> MFIKPGRCPKPAVQEDFDAARYLGVWYDIQRLPNKFQKGECATATYSLSPGVGFSVFNRERLANGTIKSVIGSAIAEDPCEPAKLQFFHENAAPVPYWVLSTDYDNYALVYSCINEGASHAAYASIVSRQPTLPEETIKKLQGTMSSFGVGVDTLLTTNQDAAYCSAMNQKLAA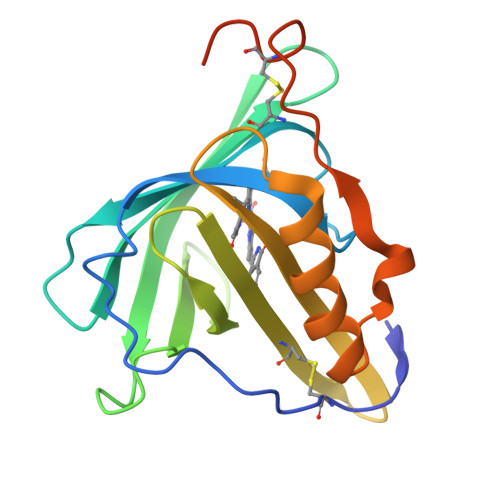ALEHHHHHH> XXXXXXXXXXXXXXXXXX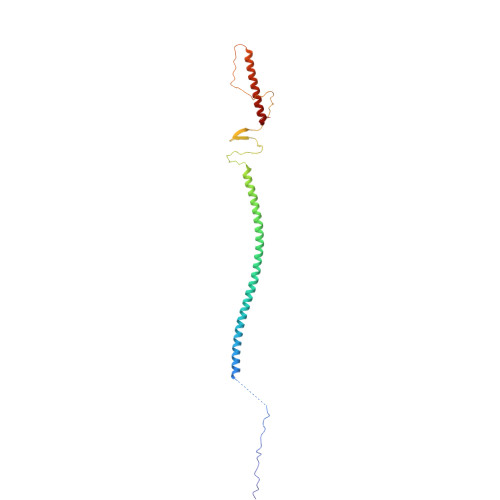XXXAYDAQVKNDEQDVELADHDARIAANTKAINILEVRLTTAEGKIVVLRSDVDYLLDEVIDIQAHLVTVDQRLDGVESDVSDIKSDYVSKTVTESQSLASPLDVKTSYSVDGIQVVGARQTGWTAATGTPLLGSFNANQSYTVGTTYTQSEVAALATGLEQARQRILALETALRLHGLID> MRGSHHHHHHGMASMNEFPVVLVINCGSSSIKFSVLDVATCDVLMAGIADGMNTENAFLSINGDKPINLAHSNYEDALKAIAFELEKRDLTDSVALIGHRIAHGGELFTQSVIITDEIIDNIRRVSPLAPLHNYANLSGIDAARHLFPAVRQVAVFDTSFHQTLAPEAYLYGLPWEYFSSLGVRRYGFHGTSHRYVSRRAYELLDLDEKDSGLIVAHLGNGASICAVRNGQSVDTSMGMTPLEGLMMGTRSGDVDFGAMAWIAKETGQTLSDLERVVNKESGLLGISGLSSDLRVLEKAWHEGHERARLAIKTFVHRIARHIAGHAASL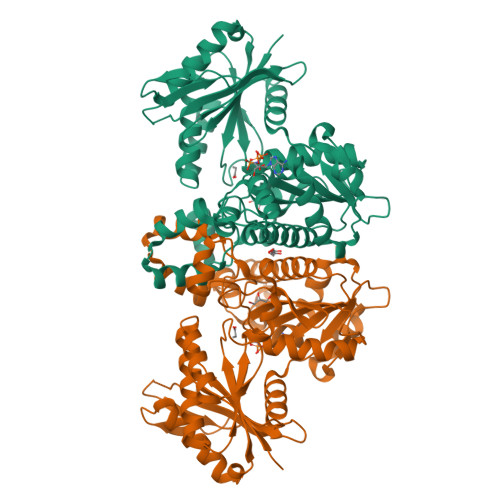HRLDGIIFTGGIGENSVLIRQLVIEHLGVLGLTLDVEMNKQPNSHGERIISANPSQVICAVIPTNEEKMIALDAIHLGNVKAPVEFA> EQCGRQAGGKLCPNNLCCSQWGWCGSTDEY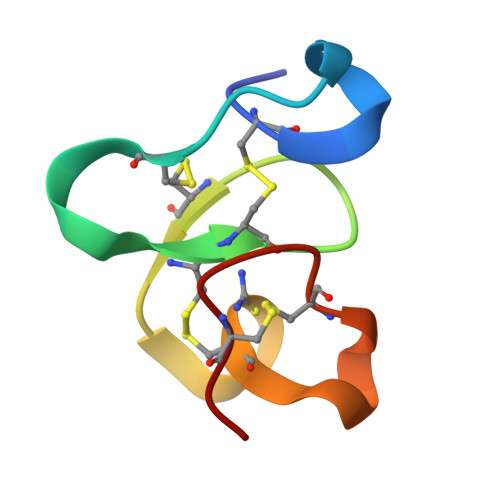CSPDHNCQSNCKD> DKATIPSESPFAAAEVADGAIVVDIAKMKYETPELHVKVGDTVT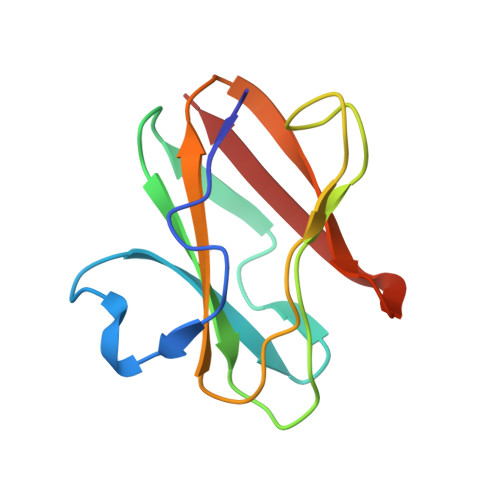WINREAMPHNVHFVAGVLGEAALKGPMMKKEQAYSLTFTEAGTYDYHCTPHPFMRGKVVVE>[2x]EVTIEAVPPQVAEDNNVLLLVHNLPLALGAFAWYKGNTTAIDKEIARFVPNSNMNFTGQAYSGREIIYSNGSLLFQMITMKDMGVYTLDMTDENYRRTQATVRFHVHQPVTQPFLQVTNTTVKELDSVTLTCLSNDIGANIQWLFNSQSLQLTERMTLSQNNSILRIDPIKREDAGE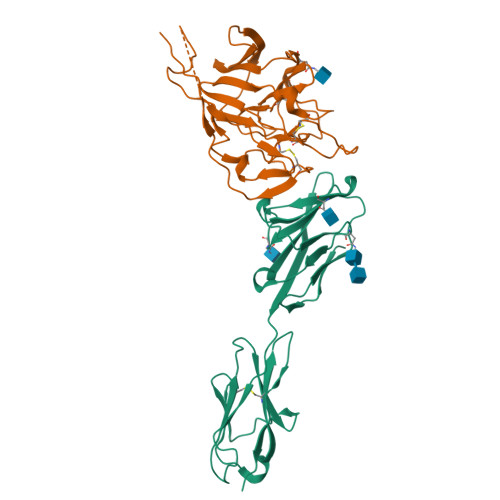YQCEISNPVSVRRSNSIKLDIIFDPHHHHHH;>[2x]YIGDFRCIQLVNSNGANVSAPSISTETVEVSQGLGTYYVLDRVYLNATLLLTGYYPVDGSKFRNLALTGTNSVSLSWFQPPYLSQFNDGIFAKVQNLKTSTPSGATAYFPTIVIGSLFGYTSYTVVIEPYNGVIMASVCQYTICQLPYTDCKPNTNGNKLIGFWHTDVKPPICVLKRNFTLNVNADAFYFHFYQHGGTFYAYYADKPSATTFLFSVYIGDILTQYYVLPFICNPTAGSTFAPRYWVTPLVKRQYLFNFNQKGVITSAVDCASSYTSEIKCKTHHHHHH>MPFIYRRRVQFYETDAQGIVHHSNYFRYFEEARGEFLRSKGFPYSKMRDMGLEVVLLNAYCEYKKPLFYDDVFEVHLNLE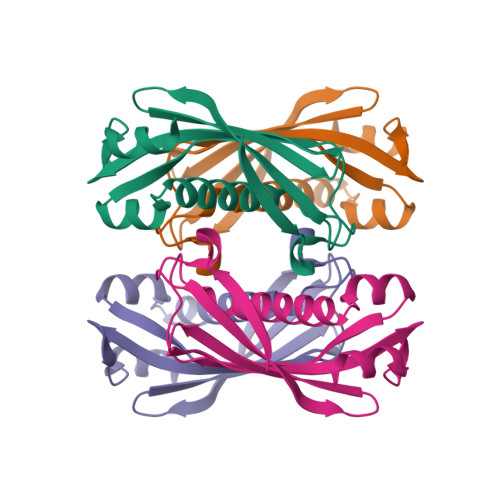ELSRFTFTFSYIVFKEDIAVAKANTKHCMVKNGKIVSIPKEVLEVLKD[2x]> GDNQDRTVANTQPSGPSNSKEIPALTAVETGHTSQVDPSDTLQTRHVVNFHSRSESTVENFMGRAACVFMDQYKLNGEETSTDNFAVWTINVREMAQLRRKCELFTYMRFDIEMTMVITSCQ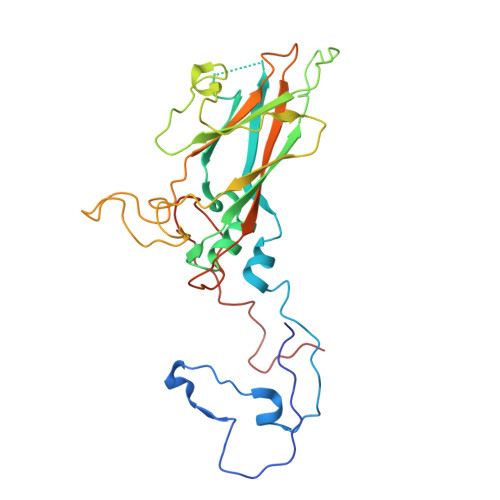DQGTQLEQDMPVLTHQIMYVPPGGPIPAKVDSYEWQTSTNPSVFWTEGNAPARMSIPFISVGNAYSLFYDGWSHFTQDGTYGYTTLNAMGKLFVRHVNKSSPHQITSTIRVYFKPKHIKAWVPRPPRLCPYINKGDVNFVVTEVTDARKSITDTPH>MELIRIAMRKDLENDKSLMSKWAAVAGLKNPNPLYDFLNHDGKTFSEFNSIVNIVKTHYPDQEYELMENYCLLLDPNTKAARSALEYADANSFNTLTDKLVEKMSIASNLKSKEYGKIYEIHRKLSRGEIDVLEASKNIGKYRIKTDEMNIFSKMIPMYDYLSKGNFSPMKSLLKQIDLNDIKENNYLKKSFETRIYVLLSNIYLNENELELSRKYAEKAIKSTDTKRFLVFSYLTIGTSYIFSDYALSKQNYLSGYEIAKGNSV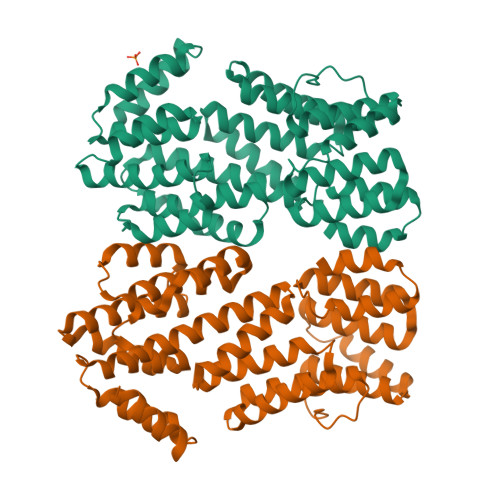FEEFFKRNLSFLNNFWNKENPWINYDSNAVTDVQEVIFELINQKKLERALTLLKSLERKKQNENDLGFHYYLEGLITNDKEAFYKSVEYFKLSQDKLFIKMPLIKLESLGENPRLLKIISM[2x]> GAMAHIIILKSMNATFETKFLVVPFKPDGLKLGRPVTNSVNKNNSGSKRDLFSQQVRPDNGNFDSRVLSRNHACLSCDPTSGKIYIRDLKSSNGTFVNGVK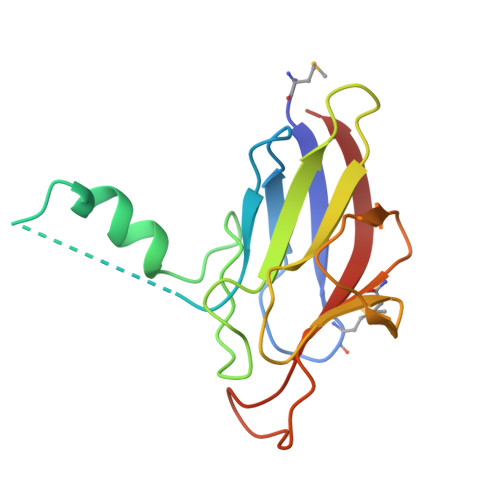IRQNDVELKVGDMVDLGTDIDSKFEHRKISAYVEEISVI> MFIYYKRTKQGSTEQWFVIGGKRIYLPTMTYVNEANDLIKRYGGNTNVTTYNHD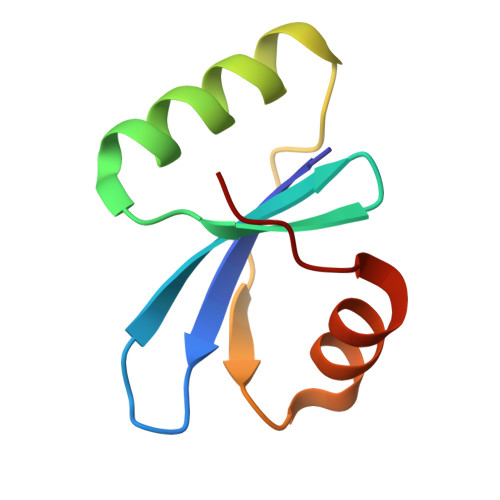NFGLKMMEAALPQVKV>[2x]QGGAAAPISSHCRLDKSNFQQPYITNRTFMLAKEASLADNNTDVRLIGEKLFHGVSMSERCYLMKQVLNFTLEEVLFPQSDRFQPYMQEVVPFLARLSNRLSTCHIEGDDLHIQR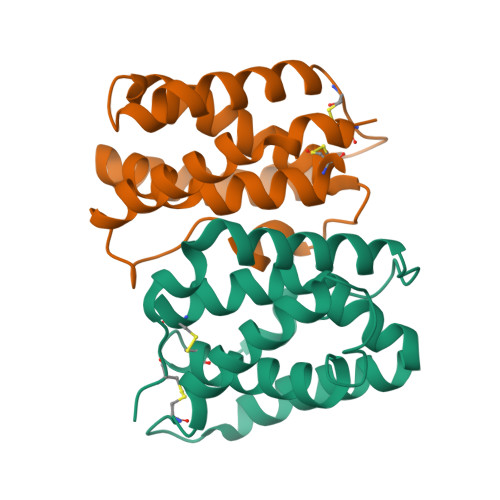NVQKLKDTVKKLGESGEIKAIGELDLLFMSLRNACI>[2x]MEELEQGLLMQPWAWLQLAENSLLA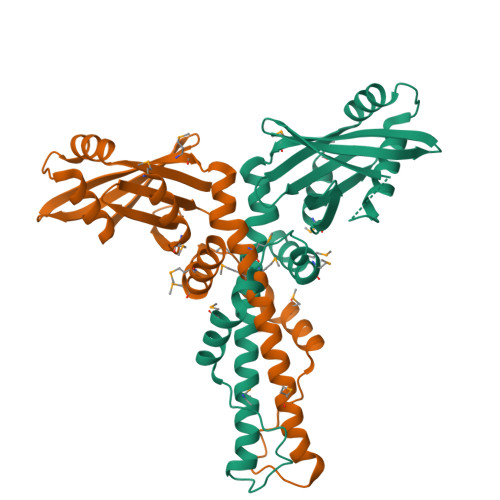KVFITKQGYALLVSDLQQVWHEQVDTSVVSQRAKELNKRLTAPPAAFLCHLDNLLRPLLKDAAHPSEATFSCDCVADALILRVRSELSGLPFYWNFHCMLASPSLVSQHLIRPLMGMSLALQCQVRELATLLHMKDLEIQDYQESGATLIRDRLKTEPFEENSFLEQFMIEKLPEACSIGDGKPFVMNLQDLYMAVTTQHHHHHH>MAEIYRKSAAETFTQLEATEKGLTTSEVTKRQEKYGFNELKNKKKGGGGDPLWKLFLETFKDPMVIVLVIAALVQLVLGEVVESLIIFLVLIVNSIISVVQTRKAESSLDALREMSAPVAKVIRDGSKQSIHARELVPGDVVILDAGDFVPADGRLFESGSLKIDEGMLTGESEAVEKYIDTIPDEVGLGDRVNMVFSGSLVVYGRGMFVVTGTASETEIGKIAGLLETAEAKQTPLQRKLESFSKKLGLGILALCVLIFAVEAGRVLLGDNSADMATAILNAFMFAVAVAVAAIPEALSSIVTIVLAVGTNKMAKQHAIIRKLPAVETLGSTSVICTDKTGTLTQNKMTVVDYYLPDGTKENFPESPENWSEGERRLIHIAVLCNDSNINSEGKELGDPTEVALIAFSNKNNQDYNEIREKFIREGEIPFDSDRKLMSTLHTFNENKAMLTKGGPDVMFARCSYVFLDGEEKPMTEEILAKLKETNEEFSNQALRVLAYGYKRMPADTTELKLEDEQDIVLVGLTAMIDPPREAVYASIEESKKAGIRTVMITGDHKTTAQAIGRDIGLMDADDIALTGQELDAMPEEELDKKLEHIAVYARVSPENKIRIVKAWQKKGKITAMTGDGVNDAPALKQADIGVAMGSGTDVAKDSAAMILTDDNFVSIVDAVGVGRTVFDNIKKSIAYL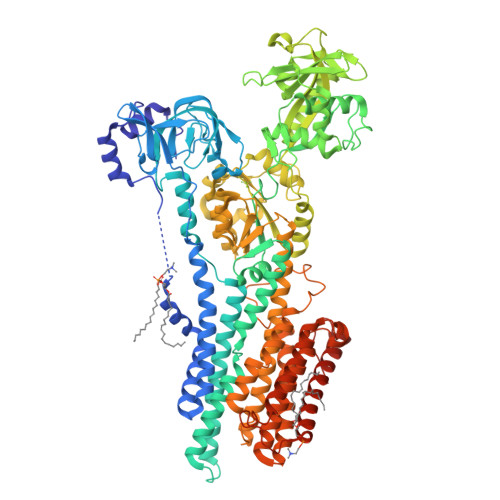FAGNLGAIIAILFALVLDWINPFTALQLLFINLVNDSLPAIALGMEKAEPDVMKRKPRDINEGIFAGGTMRAVISRGVLIGIAVIISQYIGMQISPEMSVAMAFTTLILARTLQTFAARSNVQTAFGAGFFSNKYVIGAVLLCFVLYGITVLPGAREIFSIPASFGLHEWSIAAGLALAAVVMMEIIKVVQNKFFKDYDIPTTENLYFQGLEHHHHHHHHHH[8x]>[4x]MAKNIQAIRGMNDYLPGETAIWQRIEGTLKNVLGSYGYSEIRLPIVEQTPLFKRAIGEVTDVVEKEMYTFEDRNGDSLTLRPEGTAGCVRAGIEHGLLYNQEQRLWYIGPMFRH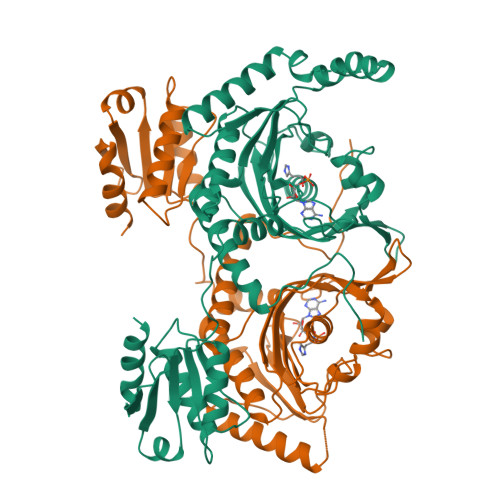ERPQKGRYRQFHQLGCEVFGLQGPDIDAELIMLTARWWRALGISEHVTLELNSIGSLEARANYRDALVAFLEQHKEKLDEDCKRRMYTNPLRVLDSKNPEVQALLNDAPALGDYLDEESREHFAGLCKLLESAGIAYTVNQRLVRGLDYYNRTVFEWVTNSLGSQGTVCAGGRYDGLVEQLGGRATPAVGFAMGLERLVLLVQAVNPEFKADPVVDIYLVASGADTQSAAMALAERLRDELPGVKLMTNHGGGNFKKQFARADKWGARVAVVLGESEVANGTAVVKDLRSGEQTAVAQDSVAAHLRTLLG> MGVYDYKNFGTADSKALFSDAMAITLYSYHNLDNGFAAGYQHNGFGLGLPATLVTALLGGTDSQGVIPGIPWNPDSEKLALDAVKKAGWTPITASQLGYDGKTDARGTFFGEKAGYTTAQVEILGKYDAQGHLTEIGIAFRGTSGPRENLILDSIGDVINDLLAAFGPKDYAKNYVGEAFGNLLNDVVAFAKANGLSGKDVLVSGHSLGGLAVNSMADLSGGKWGGFFADSNYIAYASPTQSSTDKVLNVGYENDPVFRALDGSTFTGASVGVHDAPKESATDNIVSFNDHYASTAWNLLPFSILNIPTWISHLPTAYGDGMNRIIESKFYDLTSKASTIIVANLSDPARANTWVQDL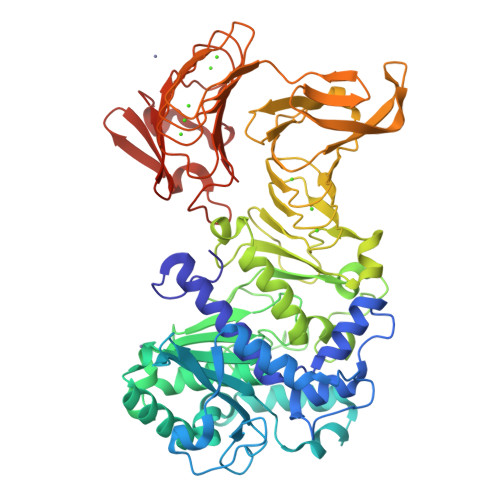NRNAETHKGSTFIIGSDSNDLIQGGSGNDYLEGRAGNDTFRDGGGYNVILGGAGNNTLDLQKSVNTFDFANDGAGNLYVRDANGGISITRDIGSIVTKEPGFLWGLFKDDVTHSVTASGLKVGSNVTQYDASVKGTNGADTLKAHAGGDWLFGLDGNDHLIGGVGNDVFVGGAGNDLMESGGGADTFLFNGAFGQDRVVGFTSNDKLVFLGVQGVLPNDDFRAHASMVGQDTVLKFGGDSVTLVGVALNSLSADGIVIA(2~{S},3~{S},4~{S},5~{R},6~{S})-3,4,5-tris(oxidanyl)-6-[(1~{R})-6'-oxidanyl-3-oxidanylidene-spiro[2-benzofuran-1,9'-xanthene]-3'-yl]oxy-oxane-2-carboxylic acid | C26 H20 O11 | 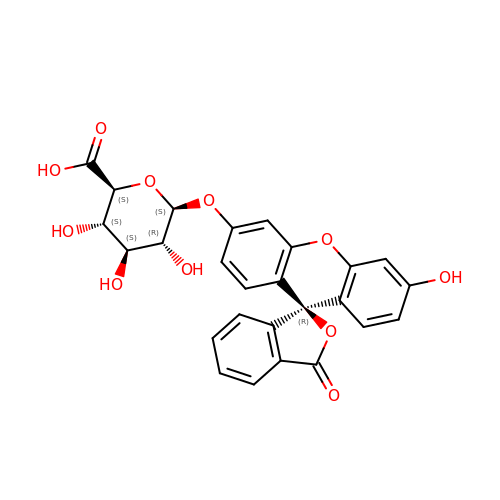RSSKCAKCONQQRX-MDPQNUMESA-N>[2x]MNLKDKILGVAKELFIKNGYNATTTGEIVKLSESSKGNLYYHFKTKENLFLE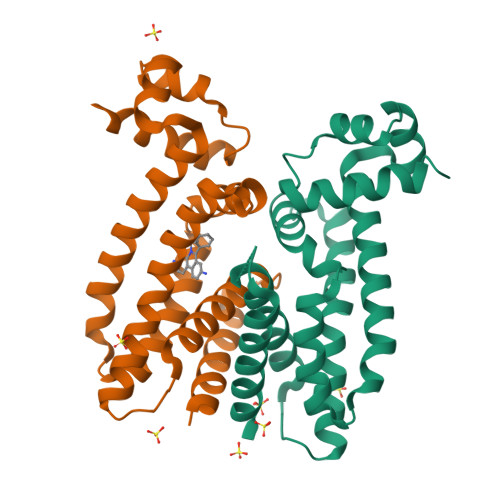ILNIEESKWQEQWKSEQIKAKTNREKFYLYNELSLTTQYYYPLQNAIIEFYTEYYKTNSINEKMNKLENKYIDAYHVIFKEGNLNGEWSINDVNAVSKIAANAVNGIVTFTHEQNINERIKLMNKFSQIFLNGLSKHHHHHH>[2x]MSKVPSDIEIAQAAKMKPVMELARGLGIQEDEVELYGKYKAKISLDVYRRLKDKPDGKLILVTAITPTPAGEGKTTTSVGLTDALARLGKRVMVCLREPSLGPSFGIKGGAAGGGYAQVVPMEDINLHFTGDIHAVTYAHNLLAAMVDNHLQQGNVLNIDPRTITWRRVIDLNDRALRNIVIGLGGKANGVPRETGFDISVASEVMACLCLASDLMDLKERFSRIVVGYTYDGKPVTAGDLEAQGSMALLMKDAIKPNLVQTLENTPAFIHGGPFANIAHGCNSIIATK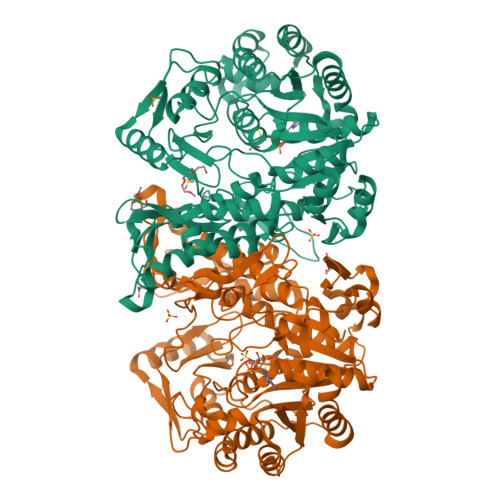TALKLADYVVTEAGFGADLGAEKFYDVKCRYAGFKPDATVIVATVRALKMHGGVPKSDLATENLEALREGFANLEKHIENIGKFGVPAVVAINAFPTDTEAELNLLYELCAKAGAEVALSWAKGGEGGLELARKVLQTLESRPSNFHVLYNLDLSIKDKIAKIATEIYGADGVNYTAEADKAIQRYESLGYGNLPVVMAKTQYSFSDDMTKLGRPRNFTITVREVRLSAGGRLIVPITGAIMTMPGLPKRPAACNIDIDADGVITGLF>[4x]MSLSDRVKKIESFTLTLPRETPYLGKPRPGEEPNGRGYLVRKANRTVYPTFDRSVLVRIETENGAVGWGETYGLVAPRATMEIIDDLLADFTIGRDPFDAAAIHDDLYDLMRVRGYTGGFYVDALAAIDIALWDLAGKLAGLPVCKLLGGQRRDRIAAYISGLPEDTRAKRAELAAAWQAKGFSSFKFASPVADDGVAKEMEILRERLGP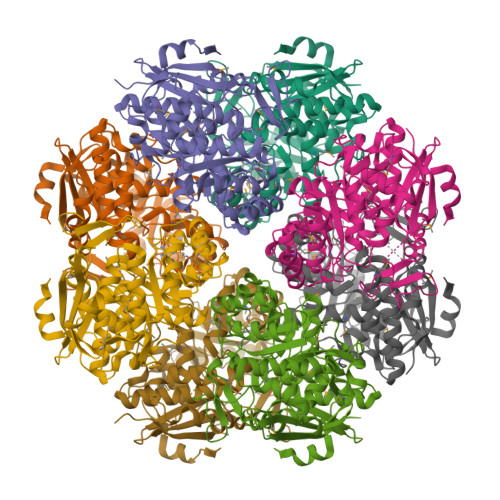AVRIACDMHWAHTASEAVALIKAMEPHGLWFAEAPVRTEDIDGLARVAASVSTAIAVGEEWRTVHDMVPRVARRALAIVQPEMGHKGITQFMRIGAYAHVHHIKVIPHATIGAGIFLAASLQASAALANVDCHEFQHSIFEPNRRLLVGDMDCLNGEYVVPTGPGLGVEPSKEAQGLLKKHEGHHHHHH>MNLVNKAQLQKMAYVKFRIQEDEYVAILNALEEYHNMSESSVVEKYLKLKDINNLTDNYLNTYKKSGRNKALKKFKEYL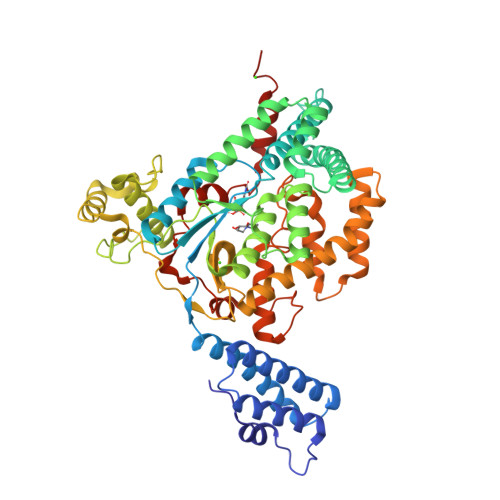TMEVLELKNNSLTPVEKNLHFIWIGGQINDTAINYINQWKDVNSDYTVKVFYDSNAFLINTLKKTIVESATNNTLESFRENLNDPEFDYNKFYRKRMEIIYDKQKHFIDYYKSQIEENPEFIIDNIIKTYLSNEYSKDLEALNKYIEESLNKITANNGNDIRNLEKFADEDLVRLYNQELVERWNLAAASDILRISMLKEDGGVYLDVDMLPGIQPDLFKSINKPDSITNTSWEMIKLEAIMKYKEYIPGYTSKNFDMLDEEVQRSFESALSSKSDKSEIFLPLDDIKVSPLEVKIAFANNSVINQALISLKDSYCSDLVINQIKNRYKILNDNLNPSINEGTDFNTTMKIFSDKLASISNEDNMMFMIKITNYLKVGFAPDVRSTINLSGPGVYTGAYQDLLMFKDNSTNIHLLEPELRNFEFPKTKISQLTEQEITSLWSFNQARAKSQFEEYKKGYFEGALGED[3x]> MGDTTQLVKEYQEKRSKLEKFMKNPQHDASLLSNSNEFRDKNVEFFASGGTRTSKFDKLENHPFLGYPYKRGVKRVIQEAQDNQSHYEPHVEAGGGEDLYGICIDIDEFSKTATIVPITNNFEGYLVAKDSTVKVKDKLIFNK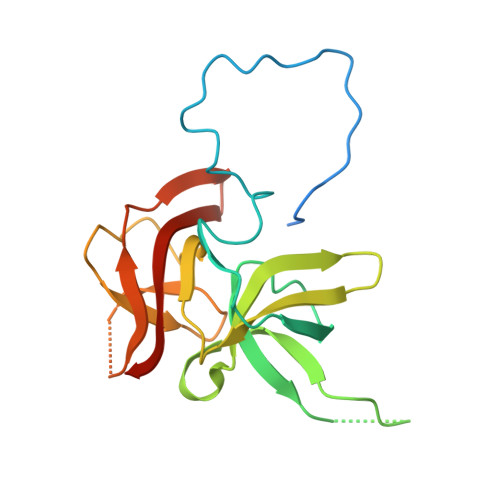DGALEKVTGAPNKATINATALTDAKQISNEVYLVKVAVFGNKAMSRN> GSDQEAKPSTEDLGDKKEGEYIKLKVIGQDSSEIHFKVK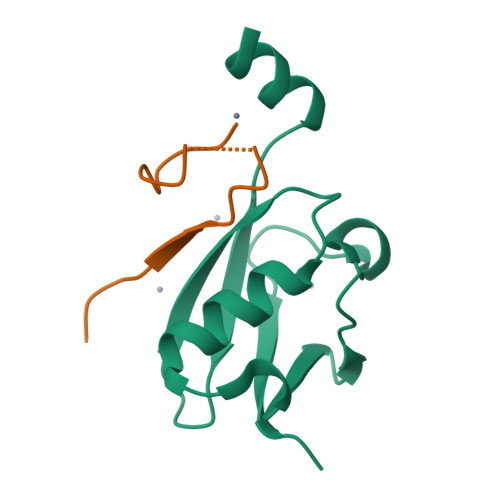MTTHLKKLKESYAQRQGVPMNSLRFLFEGQRIADNHTPKELGMEEEDVIEVYQEQTGG;> GSGAGEAEERVVVIDDDEDDDAENSSSRY>AKKKVCYYYDGDIGNYYYGQGHPMKPHRIRMTHNLLLNYGLYRKMEIYR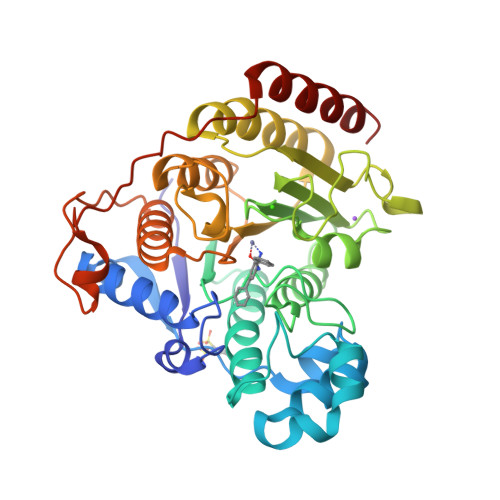PHKATAEEMTKYHSDEYIKFLRSIRPDNMSEYSKQMQRFNVGEDCPVFDGLFEFCQLSTGGSVAGAVKLNRQQTDMAVNWAGGLHHAKKSEASGFCYVNDIVLAILELLKYHQRVLYIDIDIHHGDGVEEAFYTTDRVMTVSFHKYGEYFPGTGDLRDIGAGKGKYYAVNFPMRDGIDDESYGQIFKPIISKVMEMYQPSAVVLQCGADSLSGDRLGCFNLTVKGHAKCVEVVKTFNLPLLMLGGGGYTIRNVARCWTYETAVALDCEIPNELPYNDYFEYFGPDFKLHISPSNMTNQNTPEYMEKIKQRLFENLRML[3x]> IGNNGAEKQISLHKGQPFIDTQDVGAADPNTPAVTIEGPSDYVIAIDAGTPVAPEFRDANGDKLDPSTRVTIQKCDKQGNPL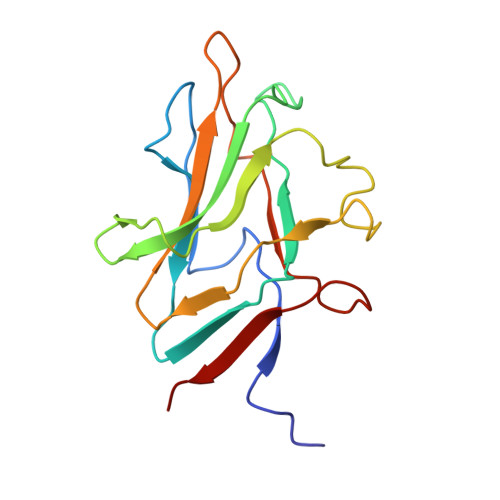GDGIVFSDTLGRFEYSKMRSDPDYMRKTTTSLMIDEREIVKIFVEVPPNANGMDADNSRITIGDDTSDYGKAVGIVEHG> PEWTYPRLSCQGSTFQKALLISPHRFGEIKGNSAPLIIREPFVACGPKECRHFALTHYAAQPGGYYNGTRKDRNKLRHLVSVKLGKIPTVENSIFHMAAWSGSACHDGREWTYIGVDGPDNDALVKIKYGEAYTDTYHSYAHNILRTQESACNCIGGDCYLMITDGSASGISKCRFLKIREGRIIKEILPTGRVEHTEECTCGFASNKTIECACRDNSYTAKRPFVKLNVETDTAEIRLM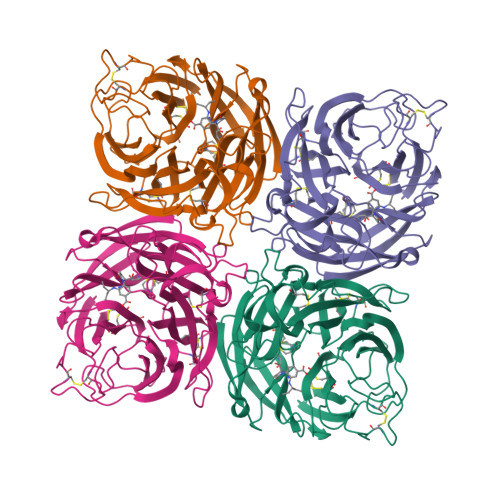CTKTYLDTPRPDDGSIAGPCESNGDKWLGGIKGGFVHQRMASKIGRWYSRTMSKTNRMGMELYVRYDGDPWTDSDALTLSGVMVSIEEPGWYSFGFEIKDKKCDVPCIGIEMVHDGGKDTWHSAATAIYCLMGSGQLLWDTVTGVDMAL> GPGSDTERPVVNVPSEITVYRGESFEYFATVTDNSNAFDLAKTVVRWLYSNQPGRGTEWLQYSVTQVGNQLKVRIFGNVPIDTTIGDYTRYVVATDAAGNVNATQTEMGNAAVDKTSVNGQFKLIIR

Many streptococci adhere to protein-attached carbohydrates expressed on cell surfaces using Siglec-like binding regions (SLBRs). Siglec-like binding regions (SLBRs) are among the streptococcal adhesive modules that bind sialoglycans. SLBRs contain two adjacent modules: a Siglec domain, which shares some features with mammalian Siglecs, and a Unique domain13 with no close homologs outside of the family. The conserved sialic acid-recognition motif governs general specificity while sequence diversity in surrounding loop regions allows the SLBR to select between related sialoglycans.

Only the crystallization conditions for SLBRHsa and the isolated Siglec domain of SLBRGspB (SLBRGspB-Siglec) supported sialoglycan binding. Distinct loops in SLBRHsa and SLBRGspB showed the largest conformational differences between the unbound and sialoglycan-bound structures. In the sTa-bound structure of SLBRGspB-Siglec, the helix of the FG loop is rotated 10° as compared to the unliganded conformation. This rotation results in a maximum physical displacement of 1.3 Å, which optimizes contacts to the GalNAc of sTa. Moreover, temperature factor analysis suggests that these loops have high flexibility in the absence of ligand.methyl (2~{R})-2-[(4~{S})-6-(4-chlorophenyl)-9-methoxy-1-methyl-4~{H}-[1,2,4]triazolo[4,3-a][1,4]benzodiazepin-4-yl]butanoate 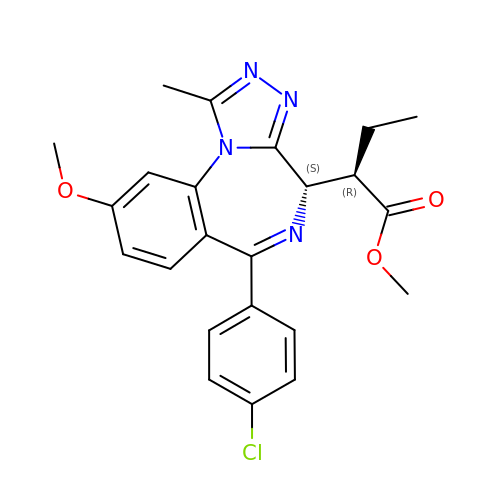| C23 H23 Cl N4 O3 | WAXCRXSIHVMWFF-UTKZUKDTSA-N>MNTDVRIEKDFLGEKEIPKDAYYGVQTIRATENFPITGYRIHPELIKSLGIVKKSAALANMEVGLLDKEVGQYIVKAADEVIEGKWNDQFIVDPIQGGAGTSINMNANEVIANRALELMGEEKGNYSKISPNSHVNMSQSTNDAFPTATHIAVLSLLNQLIETTKYMQQEFMKKADEFAGVIKMGRTHLQDAVPILLGQEFEAYARVIARDIERIANTRNNLYDINMGATAVGTGLNADPEYISIVTEHLAKFSGHPLRSAQHLVDATQNTDCYTEVSSALKVCMINMSKIANDLRLMASGPRAGLSEIVLPARQPGSSIMPGKVNPVMPEVMNQVAFQVFGNDLTITSA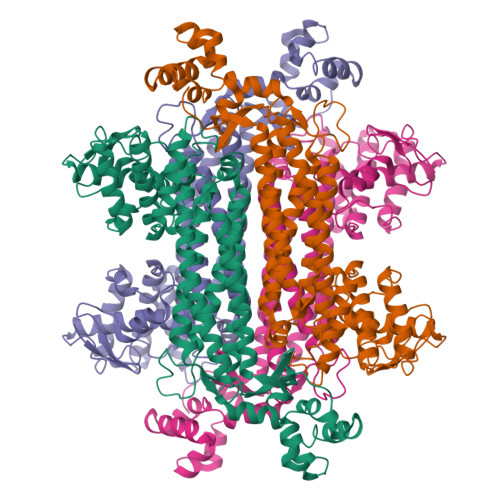SEAGQFELNVMEPVLFFNLIQSISIMTNVFKSFTENCLKGIKANEERMKEYVEKSIGIITAINPHVGYETAAKLAREAYLTGESIRELCIKYGVLTEEQLNEILNPYEMIHPGIAGRK[2x]>[12x]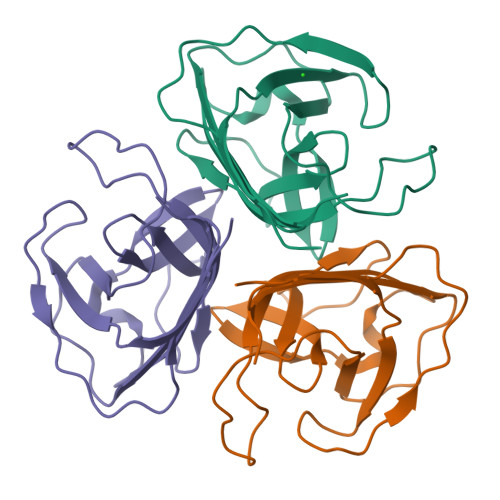MSVYGPVPTVTTRAFLPRLATAADSITSTTTTIALDPQTEQSYWTRVGDTATIHIHLVGAALPAAAPSTRIYGNFPPLRITPSSALAAQHGVIVPMQYYVAPTLPVGSSAAARIETGFIELGSLLNGAFTPLAANLIGTVGYEFAIDATYAAQ Neurexins (Nrxns) are a representative presynaptic organizer family and interact with several different postsynaptic organizers such as neuroligins (NLs), Cbln1–GluD2, and leucine-rich repeat transmembrane neuronal proteins (LRRTMs). LRRTMs are potent postsynaptic organizers that have been shown to instruct presynaptic differentiation. LRRTMs have a leucine-rich repeat (LRR) domain in the N-terminal extracellular domain, which is followed by a single transmembrane domain and a cytoplasmic region. Here, we present the crystal structures of human LRRTM2 LRR domain alone and that in complex with human Nrxn1β LNS domain at 3.15 and 3.4 Å resolutions, respectively.

We thus replaced His355 with Ala to weaken this intermolecular interaction and confirmed by SPR analyses that LRRTM2H355A and LRRTM2WT have similar affinities to Nrxin1β (–S4) (KD = 4.3 µM and 4.0 µM, respectively). We finally succeeded in the co-crystallization of Nrxn1β and LRRTM2H355A under the condition without malonate or citrate. The Nrxn1β–LRRTM2H355A complex structure was determined at 3.4 Å resolution. Nrxn1β and LRRTM2H355A form a 1:1 stoichiometric complex. However, Nrxn1β binds to the C-terminal cap of LRRTM2 with a buried surface area of 448 Å2 in the present Nrxn1β–LRRTM2 structure. A calcium ion is coordinated by the side chains of Asp141 and Asn212 and the main chains of Val158 and Ile210 in Nrxn1β (residue numbering is based on human Nrxn1β (–S4); Fig. 2b). Therefore, we concluded that LRRTM2 Glu348 interacts with the calcium ion via the coordinated water molecule. The comparison between the apo-LRRTM2T59L and Nrxn1β-bound LRRTM2H355A structures (rmsd of 0.42 Å for Cα atoms) indicates that no drastic conformational change of LRRTM2 occurs upon binding to Nrxn1β, except that the side chain of LRRTM2 Glu348 flips towards the coordinated Ca2+. Apart from the Ca2+-mediated interaction, a hydrogen bond is formed between Nrxn1β Arg206 and LRRTM2 Asp352. Phe357 of LRRTM2 hydrophobically interacts with Leu208 of Nrxn1β.

>[4x]CPPKCRCEKLLFYCDSQGFHSVPNATDKGSLGLSLRHNHITELERDQFASFSQLTWLHLDHNQISTVKEDAFQGLYKLKELILSSNKIFYLPNTTFTQLINLQNLDLSFNQLSSLHPELFYGLRKLQTLHLRSNSLRTIPVRLFWDCRSLEFLDLSTNRLRSLARNGFAGLIKLRELHLEHNQLTKINFAHFLRLSSLHTLFLQWNKISNLTCGMEWTWGTLEKLDLTGNEIKAIDLTVFETMPNLKILLMDNNKLNSLDSKILNSLRSLTTVGLSGNLWECSARICALASWLGSFQGRWEHSILCHSPDHTQGEDILDAVAGFQLCWNLSTTVTVMAGSHHHHHH;>DAASHAGTTYIFSKGGGQITYKWPPNDRPSTRADRLAIGFSTVQKEAVLVRVDSSSGLGDYLELHIHQGKIGVKFNVGTDDIAIEESNAIINDGKYHVVRFTRSGGNATLQVDSWPVIERYPAGRQLTIFNSQATIIIGGKEQGQPFQGQLSGLYYNGLKVLNMAAENDANIAIVGNVRLVGEVPGSHHHHHH[4x]>MADPGDRLGVLTTTRRVVEQAQAVWIDHDAVAQIAEAFAARQVTPPTWNRELHWSDGREALANYILVLDAVNFCFWGEPRWRIEYAGAVYDGYWALAASLKRALEQGVPLTDASYLAEITRDDVATIFAGEGEIPLLDERARILRETGSVLAERFAGRFSDAIAAAGRSAVALVDIVTNAFPSFRDVATYRGEQVRFYCRAQILVSDLYGAFDGSDLGAFDDLGELTAFADYKVPQVLHHLGILRYAPALHDRLARREEIPAGSPEEVEIRAATIWGVEELRRALA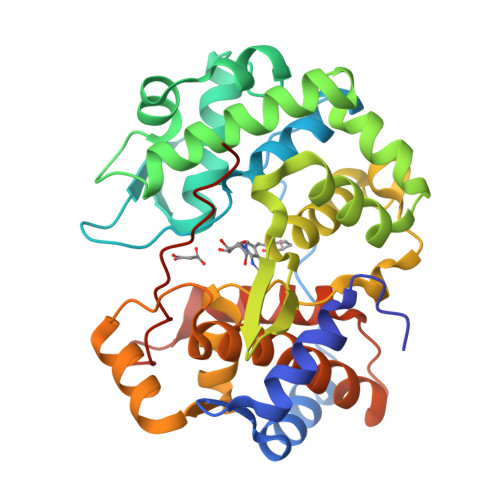SRGHALDAYQVDWLLWDEGQRLPAGTLPYHRTRTIFYLEHHHHHH[2x]>GARASVLSGGELDKWEKIRLRPGGKKQYKLKHIVWASRELERFAVNPGLLETSEGCRQILGQLQPSLQTGSEELRSLYNTIAVLYCVHQRIDVKDTKEALDKIEEEQNKSKKKAQ[39x]

During virus assembly, a primary role of the MA domain is to bring Gag to the inner leaflet (IL) of the plasma membrane via its covalently attached N-terminal myristate group and highly basic region (HBR). The MA HBR promotes Gag membrane binding by engaging in electrostatic interactions with the IL of the plasma membrane. The HIV-1 MA protein forms trimers that assemble into a hexameric lattice with central cavities at points of sixfold symmetry on PS- and PI(4,5)P2-enriched membranes. During HIV-1 maturation, the MA lattice undergoes structural rearrangement, with mature virions displaying a more regular hexameric lattice and smaller central hexameric apertures compared to their immature counterparts.

The mature WT VLPs display a regular, striated MA lattice just below the IL of the lipid bilayer (brown arrowhead) and clear lattice arrays in tomographic slices sectioning along the membrane, as previously reported. While mature WT VLPs showed the same MA localization as immature WT VLPs (IL/MA position), the mature L20K/E73K/A82T mutant VLPs displayed two separate density valleys. The density observed in the trimer center of both immature and mature WT MA lattices indicates the possible presence of a negatively charged entity that could interfere with phospholipid interaction. Specifically, the mature WT MA lattice is typically stabilized by a network of inter-trimer salt bridge interactions involving residues from the HBR and glutamates from helices 4 and 2, namely, K17-E51, R19-E51, R21-E72, and K25-E41. These salt bridges contribute significantly to the structural integrity and stability of the lattice. To assess the effects of these mutations on the mature MA lattice, we performed MD perturbation simulations on the mature MA lattices containing the R19A, R19L, E41A, and E51A mutations (simulations 10 to 13). We observe that the trimer-trimer distance distributions for all these mutants extend beyond the expected range for WT MA, differing from the WT trimer-trimer distance distribution with Jensen-Shannon distances of 0.33, 0.32, 0.18, and 0.24 for the R19A, R19L, E41A, and E51A mutations, respectively. Recent structural analysis suggests that proteolytic cleavage of SP2 from the Gag precursor by PR is required to form a mature MA lattice. The SP2 peptide was shown to bind to the inter-trimer interface, previously predicted to be a PI(4,5)P2 binding pocket, and contributes to stabilizing the mature MA lattice.>VLGKPQTDPTLEWFLSHCHIHKYPSKSTLIHQGEKAETLYYIVKGSVAVLIKDEEGKEMILSYLNQGDFIGELGLFEEGQERSAWVRAKTACEVAEISYKKFRQLIQVNPDILMRLSAQMARRLQVTSEKVGNLAFLDVTGRIAQTLLNLAKQPDAMTHPDGMQIKITRQEIGQIVGCSRFTVGRILKMLEDQNLISAHGKTIVVYGT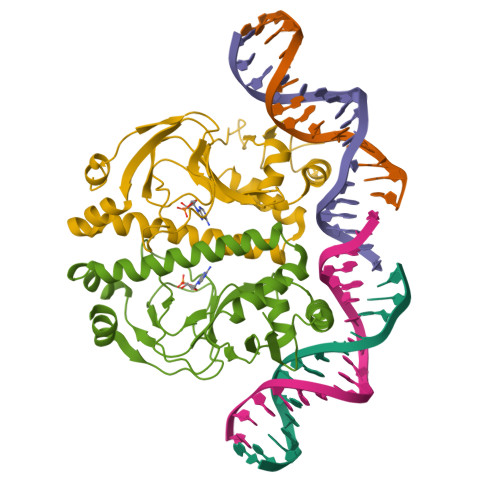R[2x]>[2x]DNKITDEQIAEWNSKQEELRDKIIRSDGDFSLSKVKYVGGFDVSYSKINHELAVSCMVVLSYPEMKQVYMNTTKVKLSCPYKSSYLAFREIEPFQQELQLLKAKK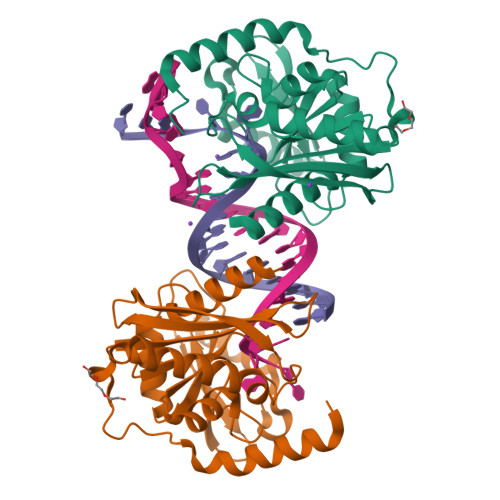PNLEPQVFLLDGNGFFHIRRCGAASHLGVLSNTRTIGVAKSLIEIPEDGVKKTEVISQFKRLRKTGGNELDIISTEKNEVLAKAVLYAPKVEKPIFVSAGHKCSLETAAKIVKGCTKTRIPEPIKMANKWSRKELKKIE>MEEPEEPADSGQSLVPVYIYSPEYVSMCDSL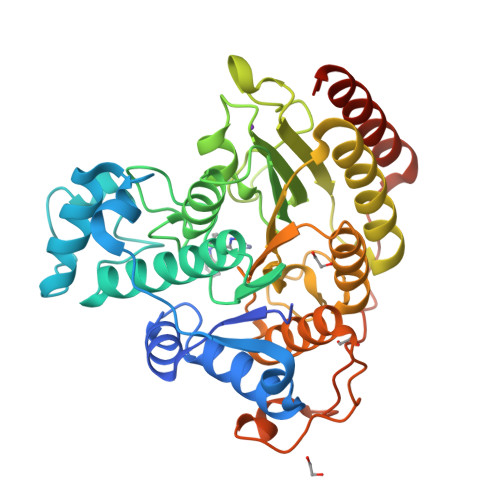AKIPKRASMVHSLTEAYALHKQMRIVKPKVASMEEMATFHTDAYLQHLQKVSQEGDDDHPDSIEYGLGYDCPATEGIFDYAAAIGGATITAAQCLIDGMCKVAINWSGGWHHAKKDEASGFCYLNDAVLGILRLRRKFERILYVDLDLHHGDGVEDAFSFTSKVMTVSLHKFSPGFFPGTGDVSDVGLGKGRYYSVNVPIQDGIQDEKYYQICESVLKEVYQAFNPKAVVLQLGADTIAGDPMCSFNMTPVGIGKCLKYILQWQLATLILGGGGYNLANTARCWTYLTGVILGKTLSSEIPDHEFFTAYGPDYVLEITPSCRPDRNEPHRIQQILNYIKGNLKHVVIEGRGSHHHHHH[2x]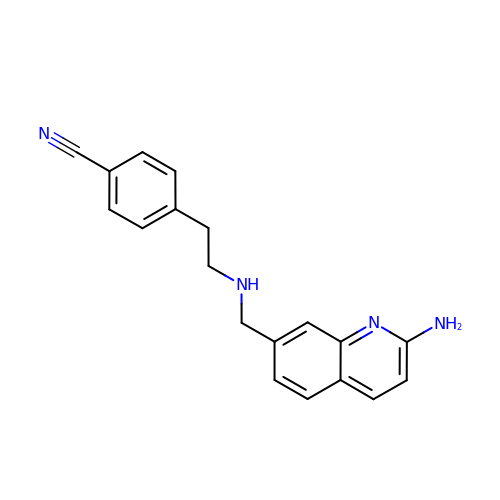4-(2-{[(2-aminoquinolin-7-yl)methyl]amino}ethyl)benzonitrile | C19 H18 N4 | CDHZAJGZCBJOTB-UHFFFAOYSA-N> MDE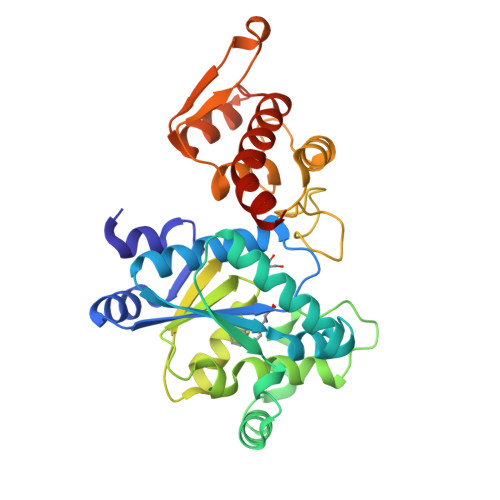FEMIKRNTSEIISEEELREVLKKDEKSALIGFEPSGKIHLGHYLQIKKMIDLQNAGFDIIILLADLHAYLNQKGELDEIRKIGDYNKKVFEAMGLKAKYVYGSSFQLDKDYTLNVYRLALKTTLKRARRSMELIAREDENPKVAEVIYPIMQVNPAHYQGVDVVVGGMEQRKIHMLARELLPKKVVCIHNPVLTGLDGEGKMSSSKGNFIAVDDSPEEIRAKIKKAYCPAGVVEGNPIMEIAKYFLEYPLTIKRPEKFGGDLTVNSYEELESLFKNKELHPMDLKNAVAEELIKILEPIRKRLLEHHHHHH> GSHMSSSPAKDPPIQRLRGAVTRCE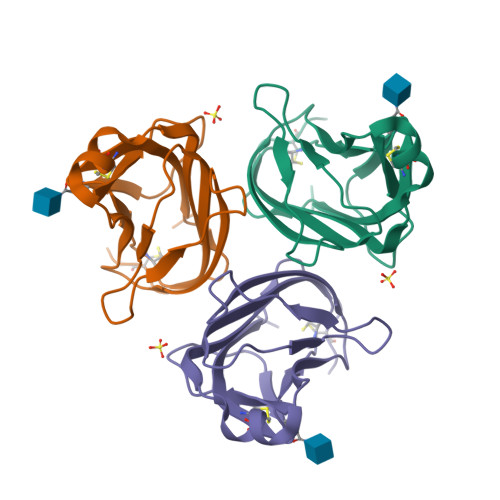DGQLFISSYKNEYQTMEVQNNSVVIKCDGLYIIYLKGSFFQEVKIDLHFREDHNPISIPMLNDGRRIVFTVVASLAFKDKVYLTVNAPDTLCEHLQINDGELIVVQLTPGYCAPEGSYHSTVNQVPL>GSHMELTPDQQTLLHFIMDSYNKQRMPQEITNKILKEAFSAEENFLILTEMATNHVQVLVEFTKKLPGFQTLDHEDQIALLKGSAVEAMFLRSAEIFNKKLPSGHSDLLEARIRNSGISDEYITPMFSFYKSIGELKMTQEEYALLTAIVILS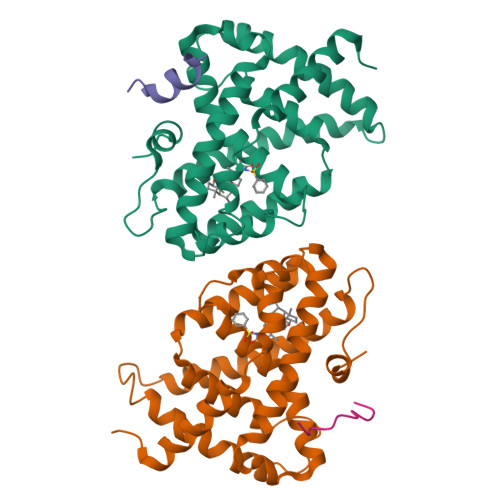PDRQYIKDREAVEKLQEPLLDVLQKLCKIHQPENPQHFACLLGRLTELRTFNHHHAEMLMSWRVNDHKFTPLLCEIWDVQ[2x];>KENALLRYLLDKD[2x]> GMTLRAAVFDLDGVLALPAVFGVLGRTEEALALPRGLLNDAFQKGGPEGATTRLMKGEITLSQWIPLMEENCRKCSETAKVCLPKNFSIKEIFDKAISARKINRPMLQAALMLRKKGFTTAILTNTWLDDRAERDGLAQLMCELKMHFDFLIESCQVGMVKPEPQIYKFLLDTLKASPSEVVFLDDIGANLKPARDLGMVTILVQDTDTALKELEKVTGIQLLNTPAPLPTSCNPSDMSHGYVTVKPRVRLHFVELGSGPAVCLCHGFPESWYSWRYQIPALAQAGYRVLAMDMKGYGESSAPPEIEEYCMEVLCKEMVTFLDKLGLSQAVFIGHDWGGMLVWYMALFYPERVRAVASLNTPFIPANPNMSPLESIKANPVFDYQLYFQEPGVAEAELEQNLSRTFKSLFRASDESVLSMHKVCEAGGLFVNSPEEPSLSRMVTEEEIQFYVQQFKKSGFRGPLNWYRNMERNWKWACKSLGRKILIPALMVTAEKDFVLVPQMSQHMEDWIPHLKRGHIEDCGHWTQMDKPTEVNQILIKWLDSDARN

To explore the utility of SX in a drug discovery setting, we selected a pharmaceutically relevant target – soluble epoxide hydro­lase (sEH) – as a model system. sEH is an enzyme that binds epoxides and converts them to their corresponding diols. The human protein is 62.5 kDa in size and consists of a C-terminal and an N-terminal domain connected by a short proline-rich linker. The C-terminal domain exhibits hydro­lase activity and the N-terminal domain is suggested to have phosphatase activity. Three residues within the C-terminal domain active site, ASP335, TYR383 and TYR466, make up the catalytic triad.

The large, potent ligands (compounds 1–4) have distinct chemical features, such as the adamatyl moiety of compounds 1 and 2, and the tetrahedral sulfur atoms of compounds 2 and 3 which are readily recognizable and could be unambiguously modelled in the electron-density maps. Interestingly, the fraction of indexed images varies between 6 and 69%, with compound 2 being the outlier on the low side. In comparison with previously published cryo-T structures of the same protein–ligand complexes, we found that the ligands generally bind in a similar fashion in the RT and the cryo-T structures.>MALDNLLRHLKISKEQITPVVLVVGDPGRVDKIKVVCDSYVDLAYNREYKSVECHYKGQKFLCVSHGIGSAGCAICFEELCQNGAKVIIRAGSCGSLQPDLIKRGDICICNAAVREDRVSHLLIHGDFPAVGDFDVYDTLNKCAQELNVPVFNGISVSSDMFYPNKIIPSRLEDYSKANAAVVEMELATLMVIGTLRKVKTGGILIVDGCPFKWDEGDFDNNLVPHQLENMIKIALGACAKLATKYAKGEFEAYVEQKLISEEDLNSAVDHHHHHH[2x]

Plasmodium purine nucleoside phosphorylase is part of the streamlined Plasmodium purine salvage pathway that leads to the phosphorylysis of both purines and 5′-methylthiopurines, byproducts of polyamine synthesis. PNP catalyzes the phosphorylytic cleavage of purine nucleosides to ribose-1-phosphate and a purine base. In P. falciparum, PfADA converts MTA to 5′-methylthioinosine (MTI), which is then converted to hypoxanthine by PfPNP. PfPNP, like Escherichia coli PNP, is hexameric and a member of the nucleoside phosphorylase family I. Unexpectedly, the PfPNP crystal structure revealed that the 5′-hydroxyl group of ImmH and 5′-methylthio group on the MT-ImmH are positioned differently in relationship to PfPNP.

Crystallographic investigation of the triple mutant PfPNP with Tyr160Phe, Val66Ile, andVal73Ile in complex with the transition state inhibitor immucillin H reveals fewer hydrogen bond interactions for the inhibitor in the hydrophobic pocket. V66I:V73I:Y160F PfPNP, a P. falciparum PNP mutant designed to mimic TgPNP, retains wild-type PfPNP efficiency with the inosine substrate, but has significantly reduced phosphorylysis of MTI. MTI is a poor substrate for the V66I:V73I:Y160F PfPNP with catalytic efficiency 160-fold lower than for inosine (9.0×104 M−1 s−1 compared to 5.6×102 M−1 s−1). ImmH binds V66I:V73I:Y160F PfPNP more than 600 times better than MT-ImmH with Ki 3.6 and 2200 nM respectively. Similar to wild-type PfPNP, V66I:V73I:Y160F PfPNP active site residues are mainly contained in one monomer with His7 and Arg45 from the adjacent subunit binding 5′-hydroxyl of ImmH and the phosphate, respectively. There is a reduction of hydrogen bonds in V66I:V73I:Y160F PfPNP to wildtype PfPNP. The Tyr160Phe mutant is unable to participate in hydrogen bonding with water and Asp206 due to the lack of the hydroxyl group on the Phe side chain. The Tyr160Phe in V66I:V73I:Y160F PfPNP cannot participate in the water-mediated interaction with the 5′-hydroxyl of ImmH due to the hydrophobic properties of the Phe160 side chain. The V66I:V73I:Y160F PfPNP pocket in the catalytic site near the 5′-hydroxyl group of ImmH is in closer proximity to CD1 of Val66Ile (4.7 Å), CD1 Val73Ile (5 Å), and CZ of Tyr160Phe (4.2 Å), than with wild-type PfPNP. In wild type PfPNP the sulfate oxygen interacts with ImmH O3′, but in V66I:V73I:Y160F PfPNP, phosphate does not seem to interact with the 3′-hydroxyl of ImmH.> MTTLLNPYFGEFGGMYVPQILMPALNQLEEAFVSAQKDPEFQAQFADLLKNYAGRPTALTKCQNITAGTRTTLYLKREDLLHGGAHKTNQVLGQALLAKRMGKSEIIAETGAGAHGVASALASALLGLKCRIYMGAKDVERQSPNVFRMRLMGAEVIPVHSGSATLKDACNEALRDWSGSYE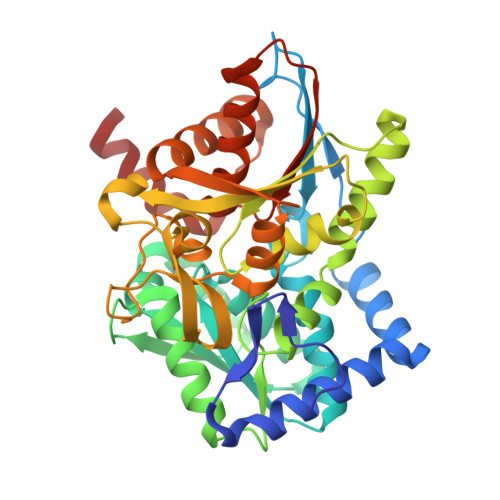TAHYMLGTAAGPHPYPTIVREFQRMIGEETKAQILDKEGRLPDAVIACVGGGSNAIGMFADFINDTSVGLIGVEPGGHGIETGEHGAPLKHGRVGIYFGMKAPMMQTADGQIEESYSISAGLDFPSVGPQHAYLNSIGRADYVSITDDEALEAFKTLCRHEGIIPALESSHALAHALKMMREQPEKEQLLVVNLSGRGDKDIFTVHDILKARE> MAHHHHHHSSGLEVLFQGPMDAPMEDAPAPVAQVKVIFTTTEPDLELPESKRQLLVPADIRRYGLSRILNSESMLDTGSIPFDFLINGSFLRSSLEDYLTSNGLSLETTLTLQYVRSLIPPVYEASFEHDDWVSAVDVLSATSPAGRWSSAANSSAAVQPGQERVLSASYDGLLRIWNASGSVIATSPSGSHGGHTASIKAAKFLTSDRLASAGMDRTVRVWKYTESDHFTGELKPTLELYGHTGSVDWLDVDGHSKHILTASADGAIGFWSASKASAPEPDASLLPGAHVSKRRKATSSVSTAQRGPLGLWSIHTAPATAAIFDPRDRTVAYSASQDHTVRTLDLTTGQVVSTLTLTHPLLSLSALTRAGTTSPLLAAGTSARHITMVDPRASSATTSVMTLRGHANKVVSLSPSPEN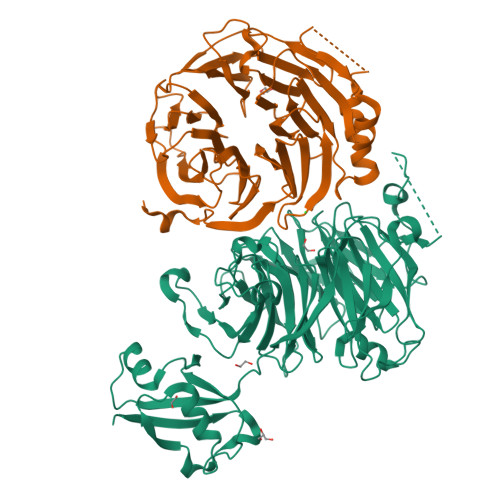EYSLVSGSHDGTCRVWDLRSVRPATKEEGSLGGVSEPVYVIERESWASKGKKKRPVAGDGCKVFSVVWDKLGIFSGGEDKKVQVNRGRNIVTEQK;> PSPDELKPFPTVQQTIFRGHEGRVRSVAIDPTGVALATGGDDGTVRVWELLTGRQVWSVKLNGDEAVNTVRWRPTKDTFILAAAAGEDIFLMIPTHPSVTPALDQASRDILNAGFGHATNGKQQANLPPGKEPPGKWARPGTRLEDEGVLLRITVRSTIKAISWHRRGDHFATVSPSGQRSSVAIHTLSKHLTQIPFRKLNGLAQTASFHPLRPLFFVATQRSIRCYDLQKLELVKIVQPGAKWISSFDVHPGGDNLVVGSYDKRLLWHDLDLSNRPYKTMRFHTEAIRAVRFHKGGLPLFADASDDGSLQIFHGKVPNDQLENPTIVPVKMLKGHKVVNKLGVLDIDWHPREPWCVSAGADGTARLWM> MNEQRSVAVWRDGAAVTVPAHQPVVTAFDLGLGRGDGIFESVAVVAGRTPHLAAHLTRLTRSAALLGLPAPGDQAWMEMVAAVLADWPAALEGVCRLFLTRGLGDGTPPTALALLAPVPADTLRQRAEGISVATLGLGVPADFRAGAPWLLGGAKTLSYAVNMAAQRHAHDLGADDVVFTSLEGRLLEGPTSTVVWAAGGTLHTPPVETGILPGTTQARLFTAAAADGWPTSVTPGTVDDLHAADAVW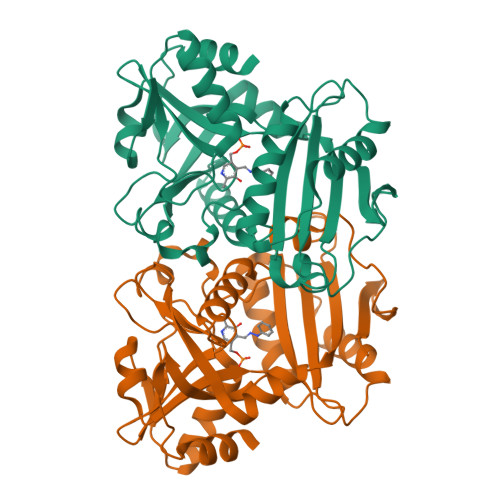LLSGVRGAAVVHTVDGVRRGDGDLSRRVRELLA> GSSHHHHHHSSGLVPRGSMSTSWSDRLQNAADMPANMDKHALKKYRREAYHRVFVNRSLAMEKIKCFGFNMDYTLAVYKSPEYESLGFELTVERLVSIGYPQELLSFAYDSTFP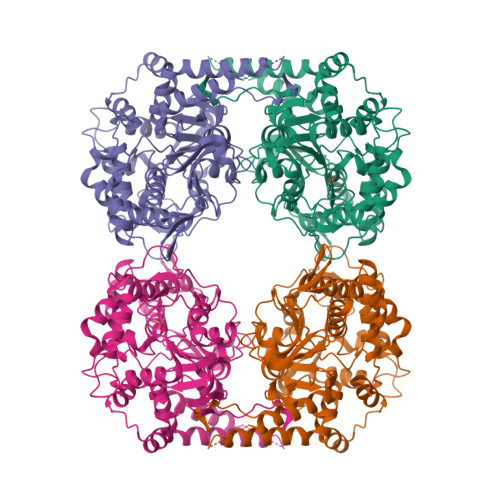TRGLVFDTLYGNLLKVDAYGNLLVCAHGFNFIRGPETREQYPNKFIQRDDTERFYILNTLFNLPETYLLACLVDFFTNCPRYTSCETGFKDGDLFMSYRSMFQDVRDAVDWVHYKGSLKEKTVENLEKYVVKDGKLPLLLSRMKEVGKVFLATNSDYKYTDKIMTYLFDFPHGPKPGSSHRPWQSYFDLILVDARKPLFFGEGTVLRQVDTKTGKLKIGTYTGPLQHGIVYSGGSSDTICDLLGAKGKDILYIGDHIFGDILKSKKRQGWRTFLVIPEFAQELHVWTDKSSLFEELQSLDIFLAELYKHLDSSSNERPDISSIQRRIKKVTHDMDMCYGMMGSLFRSGSRQTLFASQVMRYADLYAASFINLLYYPFSYLFRAAHVLMPHESTVEHTHVDINEMESPLATRNRTSVDFKDTDYKRHQLTRSISEIKPPNL>MGSSHHHHHHSSGGNENLYFQGHMARASGSERHLLLIYTGGALGMQSKGGVLVPGPGLVTLLRTLPMFHDKEFAQAQGLPDHALALPPASHGPRVLYTVLECQPLLDSSDMTIDDWIRIAKIIERHYEQYQGFVVIHGTDTMASGASMLSFMLENLHKPVILTGAQVPIRVLWNDARENLLGALLVAGQYIIPEVCLFMNSQLFRGNRVTKVDSQKFEAFCSPNLSPLATVGADVTIAWDLVRKVKWKDPLVVHSNMEHDVALLRLYPGIPASLVRAFLQPPLKGVVLETFGSGNGPSKPDLLQELRAAAQRGLIMVNCSQCLRGSVTPGYATSL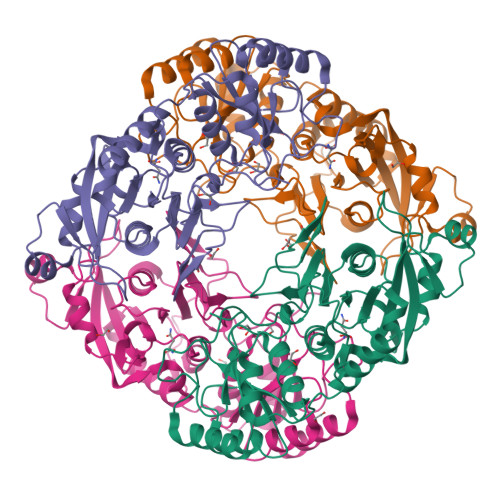AGANIVSGLDMTSEAALAKLSYVLGLPELSLERRQELLAKDLRGEMTLPTADLHQSSPPGSTLGQGVARLFSLFGCQEEDSVQDAVMPSLALALAHAGELEALQALMELGSDLRLKDSNGQTLLHVAARNGRDGVVTMLLHRGMDVNARDRDGLSPLLLAVQGRHRECIRLLRKAGACLSPQDLKDAGTELCRLASRADMEGLQAWGQAGADLQQPGYDGRSALCVAEAAGNQEVLALLRNLALVGPEVPPAI[4x]>[6x]GAMSAKEKFTSLSPAEFFKRNPELAGFPNPARALYQTVRELIENSLDATDVHGILPNIKITIDLIDDARQIYKVNVVDNGIGIPPQEVPNAFGRVLYSSKYVNRQTRGMYGLGVKAAVLYSQMHQDKPIEIETSPVNSKRIYTFKLKIDINKNEPIIVERGSVE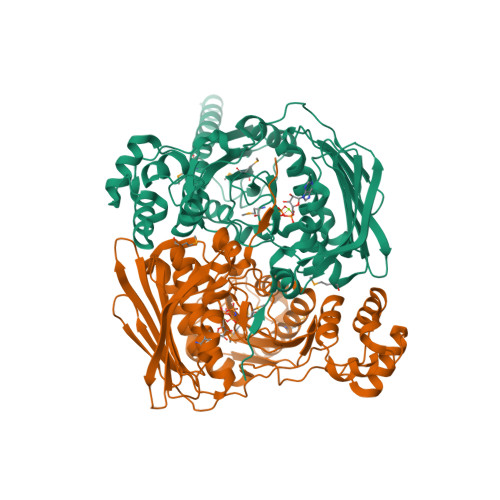NTRGFHGTSVAISIPGDWPKAKSRIYEYIKRTYIITPYAEFIFKDPEGNVTYYPRLTNKIPKPPQEVKPHPYGVDREEIKILINNLKRDYTIKEFLVNEFQSIGDTTADKILELAGLKPNKKVKNLTEEEITRLVETFKKYEDFRSPSADSLSVIGEDLIELGLKKIFNPDFAASITRKPKAYQGHPFIVEAGVAFGGSIPVGEEPIVLRYANKIPLIYDEKSDVIWKVVEELDWKRYGIESDQYQMVVMVHLCSTKIPYKSAGKESIAEVEDIEKEIKNALMEVARKLKQYLSEKRKEQEAKKKLLA Here, we report a general and rapid method for discovering α-helically constrained (Helicon) polypeptides that cooperatively induce the interaction between two target proteins without relying on previously known binders or an intrinsic affinity between the proteins. We show that Helicons are capable of binding every major class of E3 ubiquitin ligases, which are of great biological and therapeutic interest but remain largely intractable to targeting by small molecules. In addition to possessing increased stability and membrane permeability, Helicons are capable of binding large, flat protein surfaces that are inaccessible to targeting by small molecules, and Helicons have been developed to target a range of PPI targets in cells and in vivo. Characterizing Helicon-E3 co-structures and mechanisms of action, we identified new binding sites for α-helices on the E3 surfaces, as well as potential probes of the disease-linked E3, WWP123,24, highlighting the generality of our approach against this therapeutically important target class.

First, we focused on the NEDD4-like E3 ligases, which make up approximately a third of the HECT family. These include WWP1 and WWP2, which each consist of four tandem WW domains and a catalytic HECT domain at the C-terminus that transfers ubiquitin from a bound E2 first to itself and subsequently to the target substrate. The first profile (Group 1) represents Helicons such as those in cluster C71 (C71) that are pan-WWP-binders – binding indiscriminately to inactive and active forms of both HECT domains, which share ~70% sequence identity. We next solved the crystal structures of five Helicons, four in complex with WWP2HECT representing all three groups of HECT-binding clusters, and one from Group 1 with WWP1HECT. These structures revealed three distinct Helicon binding sites on WWP2HECT. In all of the structures, we found that the HECT domains adopted similarly closed (inhibited) conformations. The WWP2 proteins in the co-structures with H301, H305, and H308 share a low root-mean-square deviation (RMSD = 0.5–0.8 Å) and are shown overlaid. Group 1 Helicons H302 (WWP1HECT-binding) and H301 (WWP2HECT-binding) showed similar binding modes as each other, making contact only with the N-lobe of WWP1HECT or WWP2HECT, respectively. The Group 1 Helicons engage this same E2-binding site within WWP2HECT. Consistent with their ability to impact the catalytic activity of WWP2HECT, H301 binds near the E2 interface, while H305 and H308 may restrict the conformational change involved in activating this domain. We found that individual Helicons from all three HECT-binding Groups (1–3) could modestly inhibit the auto-ubiquitylation activity of the isolated WWP2HECT.

>[4x]GPDRSFRWKYHQFRFLCHSNALPSHVKISVSRQTLFEDSFQQIMNMKPYDLRRRLYIIMRGEEGLDYGGIAREWFFLLSHEVLNPMYCLFEYAGKNNYCLQINPASSINPDHLTYFRFIGRFIAMALYHGKFIDTGFTLPFYKRMLNKRPTLKDLESIDPEFYNSIVWIKENNLEECGLELYFIQDMEILGKVTTHELKEGGESIRVTEENKEEYIMLLTDWRFTRGVEEQTKAFLDGFNEVAPLEWLRYFDEKELELMLCGMQEIDMSDWQKSTIYRHYTKNSKQIQWFWQVVKEMDNEKRIRLLQFVTGTCRLPVGGFAELIGSNGPQKFCIDKVGKETWLPRSHTCFNRLDLPPYKSYEQLREKLLYAIEETE;>[4x]XDPADRRCIQAARVCAVLX[(2Z,6E,10E,14Z,18E,22Z,26Z)-3,7,11,15,19,23,27,31,35,39-decamethyltetraconta-2,6,10,14,18,22,26,30,34,38-decaenyl] [(2S,3S,4S,5R)-5-(hydroxymethyl)-3,4-bis(oxidanyl)oxolan-2-yl] hydrogen phosphate | C55 H91 O8 P | 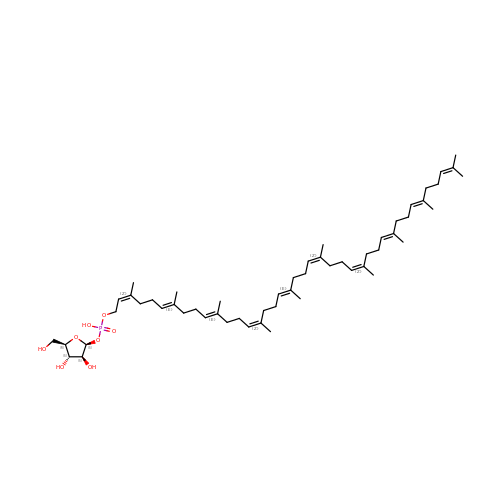YRIPSPRNAZBQAG-KAKITAEPSA-N Enolase (2-phospho-d-glycerate hydrolyase, EC 4.2.1.11) catalyzes the conversion of 2-phosphoglycerate (2-PGA) to phosphoenolpyruvate (PEP) during both glycolysis and gluconeogenesis in all three domains of life. Enolase is a metalloenzyme activated by cations of bivalent metals, such as magnesium (Mg2+). In the present study, we purified enolase-1 from Chloroflexus aurantiacus (EnoCa), a thermophilic green non-sulfur bacterium that grows photosynthetically under anaerobic conditions. Each monomer of EnoCa contains an amino terminal domain that consists of a three-stranded β-sheet packed against three α-helices and a carboxy terminal domain that consists of an eightfold α/β-barrel; both domain features are typical of the enolase superfamily.

High-resolution crystal structures were obtained for the apo protein as well as proteins with 2-PGA and PEP bound in the active site. The enolase crystals belonged to space group I4, which contained two monomers per asymmetric unit assembled into one homodimer. The structure of the apo protein and that containing 2-PGA (2-PGA EnoCa structure) of EnoCa exhibits the so-called “open” conformation, where the L1 loop is away from the active site. In the beginning of the apo EnoCa structure refinement, the difference map peaks were refined placing Mg2+(I) atom in coordination with Asp241, Glu285, and Asp313, and then three water molecules in an octahedral manner. The nature of the metal ion could not be unambiguously determined from the metal–oxygen distances of between 2.4 and 2.5 Å. Hence, the octahedral coordination sphere, the presence of Mg2+ in the crystallization buffer, and the fact that Mg2+ is the natural ligand of enolase, is consistent with the modeling of the difference density peak as an Mg2+ ion.

>[2x]MSTLIEAIVAREVLDSRGNPTIEVDVRLESGDVGRAIVPSGASTGAHEALELRDGDKSRYNGKGVLKAVQAVNEDIAEALIGFDAADQIALDQELIALDGTPNKSKLGANAILGVSLAAAKAAAAAFGLPLYRYLGGVYAHVLPVPMMNIMNGGQHATNSTDFQEFMIMPVGAESFREGLRWGAEIYHMLKKVIHDRGFSTTVGDEGGFAPSLPTNDAPLQLIMEAIEKAGYRPGEQIVIALDPATTEIFEDGKYHLKREGRSLSSAEMVDYWVDLVNRYPIISLEDGLAEDDWEGWALLRAKLGDRVQLVGDDFLVTNVQRLQRAIEAKAANSILIKLNQIGSLTETLSAIQLAQRSGWTAVVSHRSGESEDVTIADLVVATNAGQIKTGAPARTDRIAKYNQLLRIEEELGSAARYAGRSAFKV> SRMPSPPMPVPPAALFNRLLDDLGFSAGPALCTMLDTWNEDLFSALPTNADLYRECKFLSTLPSDVVEWGDAYVPERTQIDIRAHGDVAFPTLPATRDGLGLYYEALSRFFHAELRAREESYRTVLANFCSALYRYLRASVRQLHRQAHMRGRDRDLGEMLRATIADRYYRETARLARVLFLHLYLFLTREILWAAYAEQMMRPDLFDCLCCDLESWRQLAGLFQPFMFVNGALTVRGVPIEARRLRELNHIR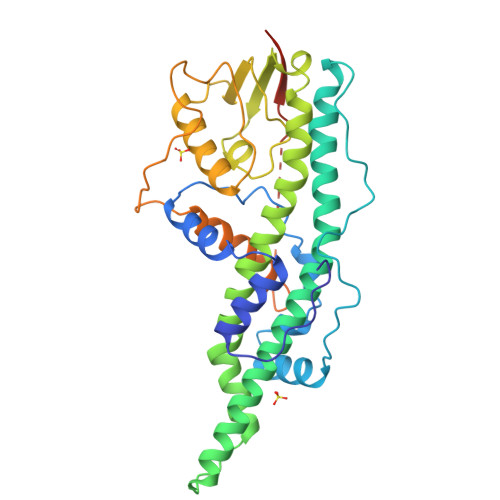EHLNLPLVRSAATEEPGAPLTTPPTLHGNQARASGYFMVLIRAKLDSYSSFTTSPSEAVMREHAYSRAPTKNNYGSTIEGLLDLPDDDAPEEAGLAAPRLSFLPAGHTRRLST The tri-longin domain (TLD) RabGEF complexes represent a family of RabGEFs with a unique conserved structural core. In each complex, two subunits that contain three longin domains (LD1 to LD3) each form a heterodimer, which is required for catalytic activity toward the cognate Rab GTPases. We here report the cryo-EM structures of the Mon1-Ccz1 and Inturned-Fuzzy core complexes bound to their cognate GTPases Ypt7 and Rab23 in the nucleotide exchange transition states, revealing a conserved catalytic mechanism with distinct modes of substrate recognition. Thus, TLD RabGEFs rely on both conservation and variability in the switch 1 regions of their substrates to realize catalytic efficiency and specificity.

Mon1-Ccz1 is a dimer in yeast and activates the Rab7 homolog Ypt7. To investigate potential interactions of Mon1NTD and Ypt7HVD with the TLD GEF core complex, we use full-length Mon1 and Ypt7 in the current study. Analysis of purified complexes by cryo-EM revealed a mixture of dimeric CtMon1-Ccz1 and trimeric CtMon1-Ccz1-Ypt7 particles. The experimental map does not reveal unmodeled density that could be interpreted as the Mon1NTD or Ypt7HVD. Consequently, our structures do not provide support for models that suggest an autoinhibitory interaction of the NTD of Mon1 with the longin domains or recognition of the Ypt7HVD by Mon1-Ccz1 at the chosen conditions. The analysis of the electrostatic surface potential of Mon1-Ccz1 revealed a large basic patch on the Mon1LD2 located opposite of the Ypt7 binding site that—together with an amphipathic helix in a disordered region of Ccz1LD2 (17)—mediates binding of Mon1-Ccz1 to model membranes. Here, the titration of CtMon1-Ccz1 on the SLBs yielded an apparent dissociation constant KD of 67 nM. With respect to membrane recruitment, we observe a notable difference between the fungal Mon1-Ccz1 complexes, which strongly bind to charged lipids, and the metazoan Mon1-Czz1-Bulli homologs, which only bind weakly. Also, while the electrostatic interactions of the fungal complexes are primarily mediated by the Mon1 subunit, metazoan complexes depend on Bulli/RMC1 for membrane association in vitro and functionality in animals.

> GPLGSMTQNNAPESVAAEGTVAGQQTDTTKPEPSSQPAPEPPSQVTTDFPPNNKPNDVPATEPASSSPRPTEPPAPPPPKPTIALSPLDIATLTFPDGTRGTFPAPPQTSAQSVSTPSIASGHVTPQRDTDTASITSVAGTLRGVTGTAGDLASLLAGDGLGRKSKAWRVLRAQQQACGEGSGEEGEITEIEGLGLGEGMEGFERELDNIPDTLPDDERLALWKGKLKHYLILSSAGKPIWSRHGDLSLVNSTMGVVQTIISFYEGARNPLLGFTAGKVRFVILIKGPLYFVAISRLRESDAQLRAQLEALYMQILSTLTLPILTNIFAHRPSTDLRGPLQGTESLLASLADSFTKGSPSTLLSALECLRLRKSQRQAITNIFLKSRCEELLYGLLVAGGKLVSVIRPRKHSLHPSDLQLIFNMLFESGGIKGNGGENWIPLCLPAFNNTGYLYMYVSFLDDKAPDDQNQPPESSNLDASNKNSSNTPDDDLTALILISPSREAFYALQSMRTRLVSQLLSTGYLSLIRSTALSGRPSITSILPKTPLLHFLYKSRPNVQWCMSSLSSLTPPGATATETLLARRKLMSVYEELHAALHARHAHLRVVYSTADEKEGEGLACLGWSTPAFEVYCVAPGCVGRAGMAREVNRVVQWARREEERLFILGGGVF;> SMTTPVSPSPSGIIPAQLGFLAIYNPALGTTDETLEDQIVYYATASTLSQARRRHRRPRRRDRQRAQSVVKDSRPNAAGATGDSEAVAEDKDPVSKEERHERLRQIGLAQGMVEFAKSFSDGEPVDTIDTEKARVILVEVEEGWWILASIDLTRLPLPQIKTPTSSSAPPPAPNLNPLPPEPAYEYSSREVKPPSLLRADLLRAYDLFLLHHGSSLSSLLASQGRAQLVASLTRFWDHFLATWNVLLHGNPACDVFGGIKLAASGELGIGVGEEERGSGEREVLEGLVERVEGLVDVVVGRYGGPPSEKGPEEEQWLGLGGEVGEEDGAVFLGVGALDRKSLRGVVQWMEEVYVWGENAFGKPRRDLSTGHFLLGLSECSEEELTSSQANPKAIFVELKPSYQHPSRKIPPEDPQPLGKVGPELPRDHTARLRPVIYVSQPFIYILLFSEITPSPSTWPTLAESLHAQLSPLQKPLLHSTSYRPERPVVETTSSSGTTTQHQIFDLVYDTETLTLQSTIPNIPDPFPYSATTPTGHSTGQQHHQQSIWTRVEALQTHAQILAILSSGRAIPTDPSSFTHLPWEEGERTCKTARGWWIVWTRVVEHSPPDAVSLHHARDDDDNDDDASCSVLGHLRSVSSSHAAGSTSSSSGSGFGLGAIPGLGGLGGWAADGATRLAQGIGIDTRRYVEGLLTSLGR> CCGTCT;> GAACGACACAGACGGTGACTC;> TCGAGTCA;> GT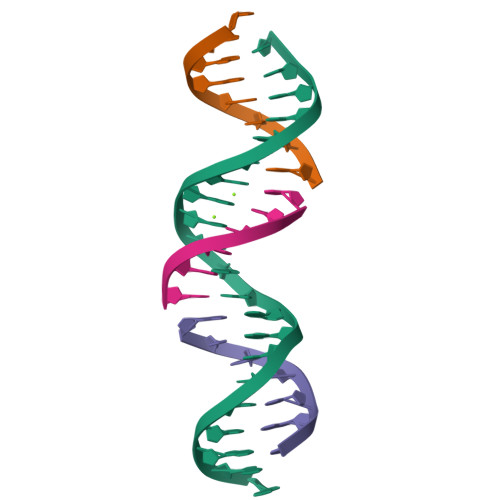GTCGT Echovirus 3 (E3), a serotype of HEV-B, first isolated in 1953, leads to highly contagious and severe diseases in humans, such as aseptic meningitis, myocarditis, and anicteric hepatitis. In line with many other HEV-Bs, E3 utilizes CD55 for viral attachment and FcRn for viral uncoating, gaining efficient entry into the host cells. Following rounds of purifications and analyses, three types of particles were identified, one containing significant amounts of viral RNA characterized as mature virus (or full particle, F-particle) and the other two being empty inside with substantially different sizes defined as expanded and compact empty particles (EE- and EC-particles). A number of key structural elements, including the VP1 BC, DE loops and C-terminus, the VP2 EF loop and VP3 EF, GH loops, contribute to the serotype-specific antigenic sites and construct the “canyon”, where many HEV receptors often bind.

Cryo-electron microscopic (cryo-EM) structures of the three types of particles: F-particle (~ 64%), EC-particle (~ 3%), and EE-particle (~ 33%) were reconstructed to 3.2 Å, 3.8 Å, and 3.1 Å resolution, respectively. By contrast, the EE-particle exhibits a typical expanded form with a ~ 4.5% increase in diameter (~ 340 Å) and notable perforations at the icosahedral two-fold axes. Superimposition of the asymmetric units (protomers) verifies the similarity in capsid structures of the F- and EC-particles and reveals substantially conformational differences between F- and EE-particles in several exposed loops, such as VP1 BC, DE, EF and HI loops, VP3 EF and GH loops. Remarkably, most of these loops are key determinants for immunogenicity in HEVs, indicating that EC-particle, rather than EE-particle, has more potential as candidates for the development of a vaccine. Incorporation of EE-particles in the vaccine would require a rational strategy to facilitate the structural transition from the expanded to the compact state. Notably, VP1 C-terminus, appearing to be the most divergent in sequence among the four subgroups in HEV-Bs, is largely disordered in the native virus structures (F-, EC-, and EE-particles), indicative of a cryptic immunogenic site, akin to the VP1 GH loop in foot-and-mouth disease virus (FMDV).

> GDVEEAIDRAVARVADTMPTGPRNTESVPALTAVETGHTSQVVPGDTMQTRHVKNYHSRTESSIENFLCRAACVYIATYKSAGGTPTERYASWRINTRQMVQLRRKFELFTYLRFDMEITFVITSTQDPGTQLAQDMPVLTHQIMYIPPGGPVPNSATDFAWQSSTNPSIFWTEGCAPARMSVPFISIGNAYSNFYDGWSHFTQEGVYGFNSLNNMGHIYVRHVNEQSLGVSTSTLRVYFKPKHVRAWVPRPPRLSPYVKSSNVNFKPTAVTTERKDINDVGTLRPVGYTNH;> GAQVSTQKTGAHETSLTASGNSTIHYTNINYYKDAASNSANRQDFTQDPSKFTEPMKDVMIKSLPALNSPTVEECGFSDRVRSITLGNSTITTQECANVVVGYGVWPSYLQDNEATAEDQPTQPDVATCRFYTLDSIQWQKESDGWWWKFPEALKNMGLFGQNMEYHYLGRSGYTIHVQCNASKFHQGCLLVVCVPEAEMGCSDVEREVVAASLSSEDTAKSFSRTESNGQHTVQTVVYNAGMGVGVGNLTIFPHQWINLRTNNSATIVMPYINSVPMDNMFRHYNFTLMIIPFAKLEYTEQASNYVPITVTVAPMCAEYNGLRLASHQ;> GLPTMLTPGSNQFLTSDDFQSPSAMPQFDVTPEMKIPGEVHNLMEIAEVDSVVPVNNTKENINSMEAYRIPVTGGDQLHTQVFGFQMQPGLNSVFKRTLLGEILNYYAHWSGSVKLTFVFCGSAMATGKFLLAYSPPGASPPQNRKQAMLGTHVIWDVGLQSSCVLCIPWISQTHYRLVQQDEYTSAGYVTCWYQTGLIVPPGAPPSCTILCFASACNDFSVRNLRDTPFIEQTQLLQ Long-range gene regulation by the DNA-binding protein KorB is important for stable vertical inheritance and horizontal transmission of the broad-host-range multidrug resistance plasmid RK2, as well as for the fitness of its host bacterium. However, in contrast to ParB, KorB also functions as a long-range silencer, repressing the expression of plasmid genes that promote replication and conjugative transfer. The best understood KorB-mediated transcriptional repression requires a 16 bp silencer sequence called OB (operator of KorB) and the small DNA-binding protein KorA that binds site specifically to a 12 bp OA sequence (operator of KorA). We find that KorB binds CTP to form a protein clamp that can entrap and slide along DNA to mediate long-range transcriptional repression, likely by allowing KorB to reach target promoters from distal OB sites.

As KorB harbours a widely distributed ParB N-terminal domain (NTD), we sought to determine whether it binds and hydrolyses CTP. Isothermal titration calorimetry (ITC) showed that KorB binds CTP with moderate affinity (KD = 4.5 ± 0.5 μM) and approximately tenfold more tightly to a non-hydrolysable analogue cytidine-5′-(3-thiotriphosphate) (CTPɣS) (KD = 0.4 ± 0.1 μM) but qualitatively much weaker to cytidine diphosphate (CDP). We then solved a 2.3 Å resolution co-crystal structure of CTPɣS with a KorB∆N30∆CTD variant that lacks the N-terminal peptide (N30) and the C-terminal domain (CTD) to locate CTP-contacting residues. Furthermore, CTP hydrolysis was abolished in the CTP-binding mutant R117A and also in the CTP-binding proficient N146A. In the presence of CTP, canonical ParB self-engages at the NTD to create a clamp-like molecule. We similarly observed dimerization of NTDs from opposing KorB subunits (with a substantial interface area of ~2,097 Å2), supporting a potential clamping mechanism. Based on the KorB∆N30∆CTD–CTPɣS co-crystal structure and sequence alignment between KorB and C. crescentus ParB, residue S47 at the NTD was substituted by cysteine on an otherwise cysteine-less KorB background. Overall, our data suggest that the ability of KorB to bind CTP and close the clamp to slide on DNA is crucial for long-range gene silencing.

>[6x]MLDSIGDLSSLLDAPAASQGGSGPIELDLDLIDEDPHQPRTADNPGFSPESIAEIGATIKERGVKSPISVRENQEQPGRYIINHGARRYRGSKWAGKKSIPAFIDNDYNEADQVIENLQRNELTPREIADFIGRELAKGKKKGDIAKEIGKSPAFITQHVTLLDLPEKIADAFNTGRVRDVTVVNELVTAFKKRPEEVEAWLDDDTQEITRGTVKLLREFLDEKKLAAALEHHHHHH The β-glycosidase from the fall armyworm Spodoptera frugiperda (Sfβgly) is an extensively studied member of glycoside hydrolase family 1 (GH1) and is an attractive template from which to gain insight on how to rationally design more efficient enzymes. The Sfβgly catalytic mechanism relies on a pair of glutamates, the proton donor E187 and the nucleophile E399, which are responsible for glycosidic bond cleavage in a double substitution mechanism. In addition to residues involved in catalysis, the active site is also composed of two sets of residues involved in the substrate binding: the highly conserved residues in the glycone-binding site (GBS) interact to the substrate glycone through hydrogen bonds and stacking interactions, while residues lining the less-conserved aglycone-binding site (ABS) modulate the Sfβgly transglycosilase activity and its preference for alkyl or glucose moieties. Sfβgly presents the typical (β/α)8 barrel fold seen for GH1 enzymes.

To obtain diffraction-quality crystals, the full-length recombinant wild-type Sfβgly lacking the signal peptide (residues 21–509) was expressed as a secreted protein in P. pastoris and purified by ion-exchange chromatography. Sfβgly crystals belong to space group P1, with 6 molecules (chains A-F) in the asymmetric unit. Although chains A, B and C present the best quality parameters, the six chains are very similar, as seen by their structural alignment and RMSD values for aligned atoms (ranging from 0.084 to 0.192 Å). The recombinant expression of Sfβgly in P. pastoris yielded a protein glycosylated at N206. We were able to model two NAG moieties at this position in chains A, B and D and only one NAG at this position in chains C, E and F, for a total of nine NAG residues. Sfβgly chains A-B, C-D and E-F form dimers in which the monomers are related by non-crystallographic pseudo-twofold symmetry. The refined Sfβgly structure presents a Tris molecule, a known β-glycosidase competitive inhibitor bound at its active site. The oxygen atoms of the carboxylate groups in the side chains of catalytic glutamates E399 and E187 are 3.9 to 4.8 Å apart from each other (as expected for retaining β-glycosidases) and hydrogen bond the Tris molecule complexed at the active site. The highly conserved glycone-binding site (GBS) is composed of residues Q39, H142, N186, W444, E451 and W452 (red), which hydrogen bond hydroxyl groups from the substrate monosaccharide and are located at the bottom of the active site (red). The aglycone-binding site (ABS) is composed of residues E190, E194, K201, W371 and M453 (blue), which are located at the entrance (top opening) of the active site (blue).

>QQRRFPDDFLFGTATASYQIEGAWDEDGKGENIWDYMVHNTPEVIRDLSNGDIAADSYHNYKRDVEMMRELGLDAYRFSLSWARILPTGMANEVNPAGIAFYNNYIDEMLKYNITPLITLYHWDLPQKLQELGGFANPLISDWFEDYARVVFENFGDRVKMFITFNEPREICFEGYGSATKAPILNATAMGAYLCAKNLVTAHAKAYYLYDREFRPVQGGQCGITISVNWFGPATPTPEDEMAAELRRQGEWGIYAHPIFSAEGGFPKELSDKIAEKSAQQGYPWSRLPEFTEEEKAFVRGTSDFFGVNHYTAFLVSATERKGPYPVPSLLDDVDTGSWADDSWLKSASAWLTLAPNSIHTALTHLNNLYNKPVFYITENGWSTDESRENSLIDDDRIQYYRASMESLLNCLDDGINLKGYMAWSLMDNFEWMEGYIERFGLYEVDFSDPARTRTPRKAAFVYKHIIKHRVVDYEYEPETMVMTIDEGH[6x]>[2x]MDIAGTTAFITGGASGIGFGIAQRLLANGARLVLADIRQDHLDEARQFFEERQQGRNVHTIRLDVSDRAQMAEAARECEAVMGGPDILINNAGIDPSGPFKDATYQDWDYGLAINLMGP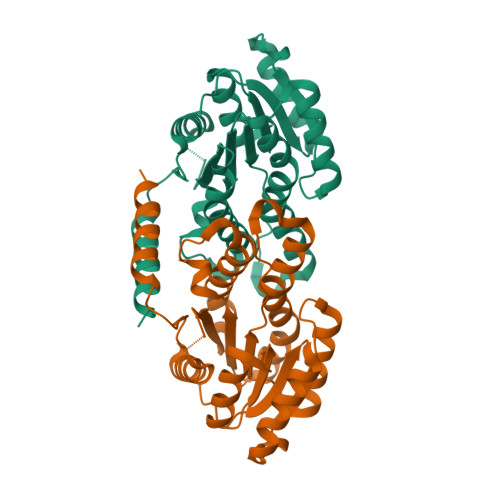INGIMAFTPGMRARGRGGHIVNTASLAGLTPMPSFMAIYATAKAAVITLTETIRDSMAEDNIGVTVLMPGPIKSRIHESGQNRPERFRAGSGLAETEQQLAKRVVADNWMEPTEVGDMIVDAIVHNKLYVSTHGNWRETCEARFQALLDSMPEARPFDFGASLAVPKEEA>GSQSSESLRCNVEPVGRLHIFSGAHGPEKDFPLHLGKNVVGRMPDCSVALPFPSISKQHAEIEILAWDKAPILRDCGSLNGTQILRPPKVLSPGVSHRLRDQELILFADLLCQYHRLDVSLP[2x];>[2x]MEDTQ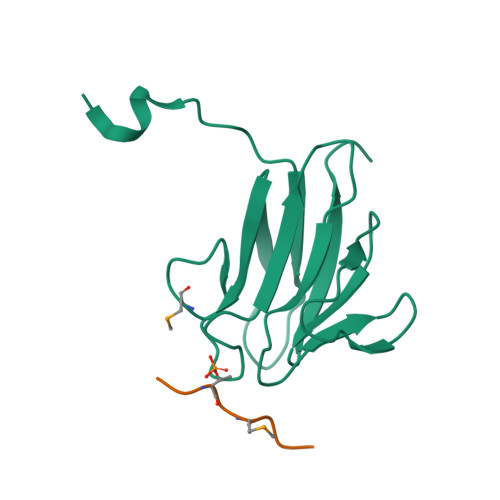MIDWD> SWDLVTCFCMKPFAGRPMIECNECHTWIHLSCAKIRKSNVPEVFVCQKCRDS;> ARTKQTARKST

PHF13, also known as Survival time associated PHD finger in Ovarian Cancer 1 (SPOC1), is a chromatin affiliated protein that is conserved from zebra fish to humans. PHF13 has been shown to modulate various processes including development, DNA damage, cell cycle, antiviral host cell response and higher order chromatin structure, underlining its biological importance. PHF13 contains a single C-terminal PHD domain, which we demonstrate biochemically and structurally, is a molecular reader of H3K4me2/3. Similar to other PHD domains, the PHD domain of PHF13 folds into a canonical Cys4-His-Cys3 (or C4HC3) motif, that coordinates two zinc ions with a well-conserved globular domain.

To gain structural insight into this specific recognition of histone H3K4me3 by the PHD domain of PHF13, we determined the crystal structures of both the apo-PHF13 PHD domain (aa 226–280) and the PHF13 PHD-H3K4me3 peptide complex. In the complex structure of PHF13 PHD-H3K4me3, we can see that the histone H3K4me3 peptide is bound against the central double-strand anti-parallel β-sheet of the PHF13 PHD domain and completes a three-stranded β-sheet. The first four residues of the H3K4me3 peptide are embedded in an exposed binding groove on the surface of the PHF13 PHD domain. Similar to other methyl lysine binding proteins, the trimethyl lysine 4 (K4me3) is bound in an aromatic cage formed by residues F241, M246 and W255 of PHF13. In addition, the K4me3 residue also forms two main chain hydrogen bonds with M246. The first residue alanine (Ala1) of the H3K4me3 peptide is anchored in a small and secluded pocket created by I247, V268, P269, E270 and F272, and the backbone amine group of Ala1 forms a hydrogen bond with the backbone carbonyl oxygen of P269 and E270 in PHF13. The limited length between the aromatic cage and the Ala1 binding pocket and the restricted nature of the Ala1 binding pocket determines that the PHF13 PHD domain selectively recognizes only methylated histone H3K4. The Arg2 residue in the H3K4me3 peptide is bound by two backbone hydrogen bonds with E248. The surface charge representation shows that Arg2 sits in a shallow negatively charged pocket, reminiscent of the Arg2 binding in the ING2 and BPTF2 PHD domain-H3K4me3 complex structures, but in contrast to the RAG2-H3K4me3 complex structure, in which Arg2 is bound in a relatively hydrophobic pocket. Our binding results show that the binding of PHF13’s PHD domain to H3K4me3 was diminished by the simultaneous asymmetric dimethylation of Arg2 (H3R2me2aK4me3).1~{H}-pyridin-2-one | C5 H5 N O | 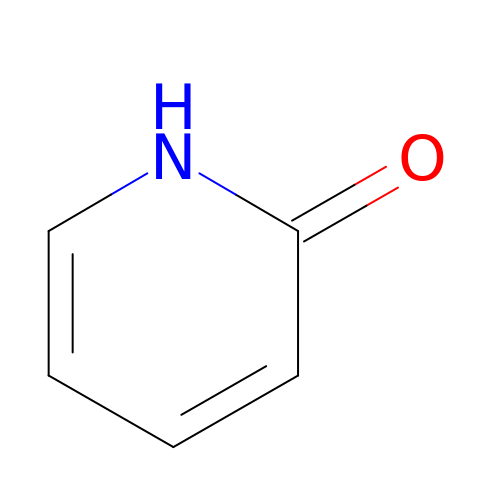UBQKCCHYAOITMY-UHFFFAOYSA-N> GAPATVTEQGEDITSKKDRGVLKIVKRVGNGEETPMIGDKVYVHYKGKLSNGKKFDSSHDRNEPFVFSLGKGQVIKAWDIGVATMKKG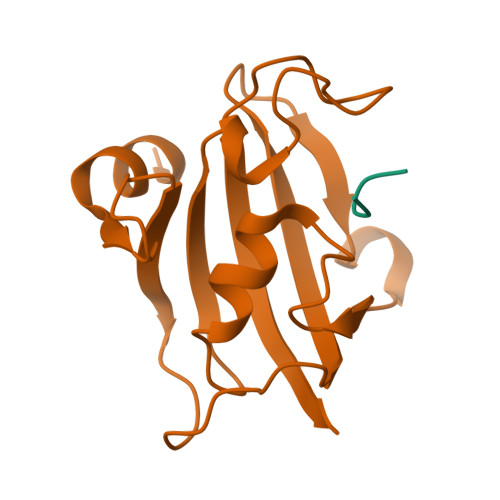EICHLLCKPEYAYGSAGSLPKIPSNATLFFEIELLDFKGE;> QFPFV> MKVYLNSMCHMAANSKTQQIQGDDNKDDKFPLASISKVVTTLWAVDRLGPDYRFKTKLHVTPTANGSYDIHIE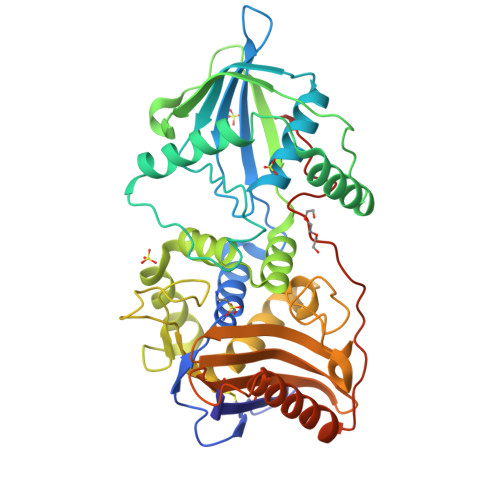GSRDPLFGRNMSYFLISELNRMKITKIEKLTFDENFLLAWLAEEKPMIGGTTPKYDTVEQQASIVRATLTSSFATAISPGYYTILKTKAARIGVQMSNRPKIDVRTISFVKKAEFQKNEKSTTMVLMSAPLKTILKRMNNQSNNYIADNLYWNLGGTEAFNAYIAGKMQADTSDIEFHNGSGNNEGSVAKPVYNEATCEMMIKVLYSLDKSLSAKGYDLSDVMAVAAKDKASTVGSYGGVMAGSTTAKTGSVNKAKTLMGSVSTKNGEIYFAVLMHTDYDKSRSDWGVASQQIKNKVSQLINQNGGPKAIKYTEQLPLPFDKYSYLTKANTITTEKKLEHHHHHH> DDDDKMLEVLFQGPGLRIVWVDEMQFQLQSFFDYIVG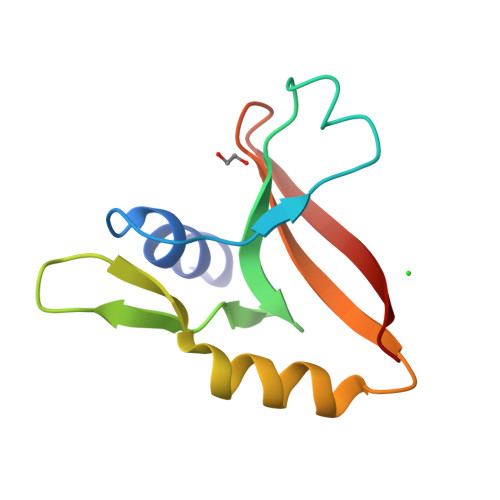FNDDPVPVVSNQHGFSYPDYRRITSIFNEHCGRTLKVNIWSAKGGTFRDEYISII>MSQTPIPEEYDDTRIMGYDPLIPPALLQNEIKASKKSLETVIKGRVDASRIIGGKDDRCLVIVGPCSIHDPEAALEYANRLKKISEELENDLVIIMRAYLEKPRTTVGWKGLINDPNVDNSFDINKGLRVSRKLYADLTGAVGIPIGSEMLDTISPQYFSDLLSFGAVGARTTESQLHRELASGLSFPIGFKNGTDGNVGVALDAVQASSKGHHFMGVTKNGLAAITTTKGNDHCFIILRGGKNLTNYDLQSVQSAKSAIAKSSNPNIKIMIDCSHDNSKKDYRNQPAVLEDVSRQIEAGENALMGVMIESNINEGKQSMPSGNEGKSALKYGVSITDSCVSWDTTV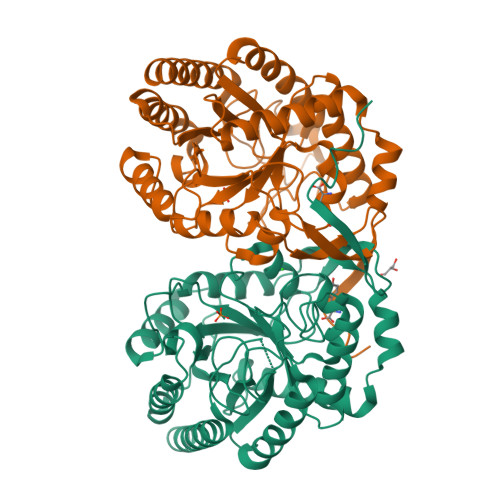KMLNNLARAVQKRRQKNGST[2x]> IPGNEKLKEKENNDSSDKATVIPNFNTTMQGSLL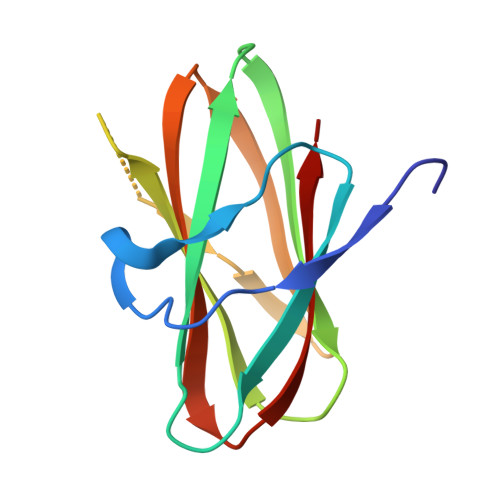GDDSRDYYSFEVKEEGEVNIELDKKDEFGVTWTLHPESNINDRITYGQVDGNKVSNKVKLRPGKYYLLVYKYSGSGNYELRVNK>SLKRLAFSSLSHTLAPFPEGELDAHLSDADFTRVFTEEDDLDLVAQSLPLVLKVYEALHLQNPAHRGLSLAVGRLYIMYANAFVQTPAQYLPEDEFEAQNEAYSRARKLYLRGARYALSSLETAYPGFTREVFSGDEQRLHKVLSRCTRVDVGTLYWVGTGYVAAFALTPLGSALPDTVHAAVMMLERACDLWPSYQEGAVWNVLTKFYAAAPESFGGGMEKAHTAFEHLTRYCSAHDPDHHITYADALCIPLNNRAGFDEALDRALAIDPESVPHNKLLVILSQKRARWLKAHVQDFFLD[3x];>[2x]GRKEKVVLKIASIAPARSIWETELKKLSAEWSEITGGLVSMKFYDMSSLGGEREGIRKLKSSRPGQAAPLDGAVFSCLGLSELAPDSGIYTLSVPFLIQNEKDLERVLHELREDLDRPFRAAGF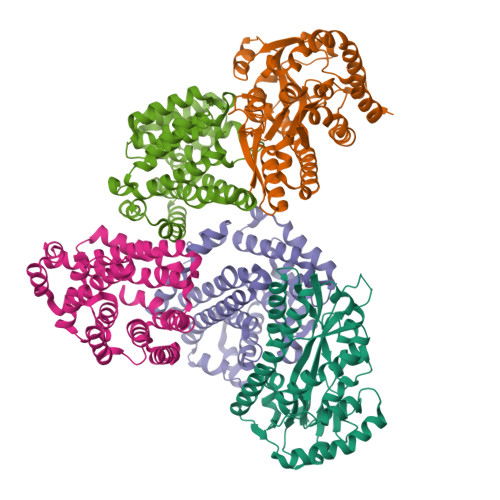RVITWTNAGWLSFYTRAPYASLGQLKKQTIALSSLDSSVLGTCFRICGFDIKDAPNVRLAPLLKAGSIDGFLSVHLFTWATGFYRYISYALDTKICPAVIGMLISDGSWARIPSRYHDAMLQAATRVRQRLANNLETLDRECSNNIQKAGVSIVHLTPQEIQEWRTEFAADVKRIQARLPGMLNMTLYEKIKHLLYSAQR> DYLLSANGSKAIDFVWSNFLKHPYNPKLKQPDANVKAAWEKHADWEHWSNMGQDWSLNTPSGLVPRPNHGIAHTLRVAQLVPVIAEFLKAYSGDPKFQKLTQKEIQKAQYMMLFSVIGRENDMSWTDANHYQQAFKEAYNGQY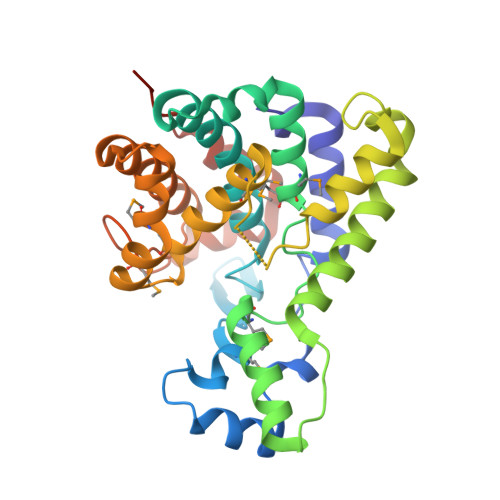SKHIYATFKENAQKGFLNHVVTNKSSLIPSLFSDESELQYWAEALDTGKPGISSASGILMALAHDLDLMRCYDKGKFNSLKMKDLVARLGGNEDAAKKLADYAHDLIVATGDRCMGYGVTQDYNYSLFGKCSLDPNECLKQLQSIPKPETTLANQYGI>[4x]GGSMLTLIQGKKIVNHLRSRLAFEYNGQLIKILSKNIVAVGSLRREEKMLNDVNLLIIVPEKKLLKHVLPNIRIKGLSFSVKVCGERKCVLFIEWEKKTYQLDLFTALAEEKPYAIFHFTGPVSYLIRIRAALKKKNYKLNQYGLFKNQTLVPLKITTEKELIKELGFTYRIPKKRL

Besides 10–23 DNAzyme, 8–17 DNAzyme can also efficiently catalyze the cleavage reaction of RNA substrate, forming the 5′-product with a 2′,3′-cyclic phosphate at the 3′-end and the 3′-product with a hydroxyl group at the 5′-end; similar structural features are also observed on the cleavage products of the naturally occurred hammerhead, hairpin, and hepatitis delta virus (HDV) ribozymes. Interestingly, the same catalytic motif of 8–17 DNAzyme has been independently isolated under different selection conditions and using different cation cofactors, indicating that this small DNAzyme is efficient and its catalytic core motif is ubiquitous in the sequence space. The central catalytic core of 8–17 DNAzyme is flankedbytwo substrate-recognizing arms, which bind to the RNA substrate via the canonical Watson–Crick base pairing. The Dz36/substrate complexes assemble into a “V” shape with two arms (P1 and P2) orientated ~70° with respect to each other in all the three structures. Unexpectedly, the catalytic core forms a compact small DNA pseudoknot consisting of two short duplexes (P3 and P4) perpendicular to each other.

Crystals of one DNAzyme/native DNA complex and DNAzyme-(2′-OMe-G) were grown in the absence of PbCl2, whereas the crystals were grown in the presence of PbCl2 for another DNAzyme/native DNA complex structure, which captured one Pb2+ ion and is referred to as DNAzyme-Pb2+ hereafter. The DNAzyme/native DNA complex without Pb2+ adopts the same space group as DNAzyme-Pb2+; as indicated by the very low value (0.307 Å) of the root mean square deviations (rmsd), the overall conformations of these two complexes are virtually identical. The conformations of the DNAzyme-Pb2+ and DNAzyme/native DNA complex without Pb2+ are virtually identical; in both structures, the N1 atom of G13 forms one hydrogen bond (H-bond, 2.8 Å) with the OP1 atom of G+1. These structural similarities indicate that the Pb2+-binding site is pre-organized and that the Pb2+ binding does not induce local and global conformational changes of this DNA catalyst. Compared to the real substrate, the G−1 residue of the native DNA lacks one hydroxyl group (O2′) at the 2′ position.>MSLVTYQTIKVRFQASVCYITFHRPEANNTINDTLIEECLQVLNQCETSTVTVVVLEGLPEVFCFGADFQEIYQEMKRGRKQASSQEPLYDLWMKLQTGPYVTISHVRGKVNAGGLGFVSATDIAIADQTASFSLSELLFGLYPACVLPFLIRRIGRQKAHYMTLMTKPISVQEASEWGLIDAFDAESDVLLRKHLLRLRRLNKKGIAHYKQFMSSLDHQVSRAKATALTANQDMFSDPQNQMGI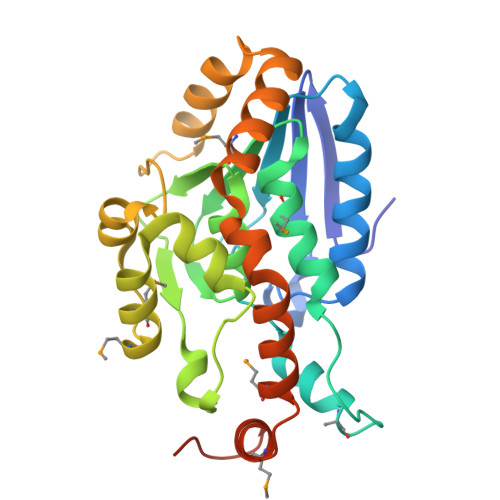IRYVETGQFPWEDQEGHHHHHH[6x]> GLIVDTRDVEERVHVMRKTKLAPTVAHGVFNPEFGPAALSNKDPRLNEGVVLDEVIFSKHKGDTKMSAEDKALFRRCAADYASRLHSVLGTANAPLSIYEAIKGVDGLDAMEPDTAPGLPWALQGKRRGALIDFENGTVGPEVEAALKLMEKREYKFACQTFLKDEIRPMEKVRAGKTRIVDVLPVEHILYTRMMIGRFCAQMHSNNGPQIGSAVGCNPDVDWQRFGTHFAQYRNVWDVDYSAFDANHCSDAMNIMFEEVFRTEFGFHPNAEWILKTLVNTEHAYENKRITVEGGMPSGCSATSIINTILNNIYVLYALRRHYEGVELDTYTMISYGDDIVVASDYDLDFEALKPHFKSLGQTITPADKSDKGFVLGHSITDVTFLKRHFHMDYGTGFYKPVMASKTLEAILSFARRGTIQEKLISVAGLAVHSGPDEYRRLFEPFQGLFEIPSYRSLYLRWVNAV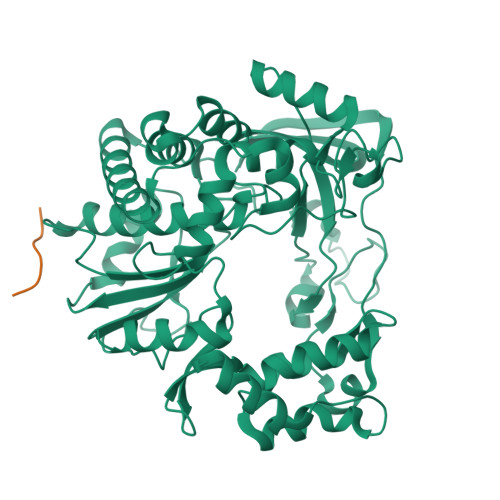CGDAAALEHHHHHH;> GPYEGPVKKPVALKVKAKNLIVTE> ETVQVNLPVSLEDLFVGKKKSFKIGRKGPHGASEKTQIDIQLKPGWKAGTKITYKNQGDYNPQ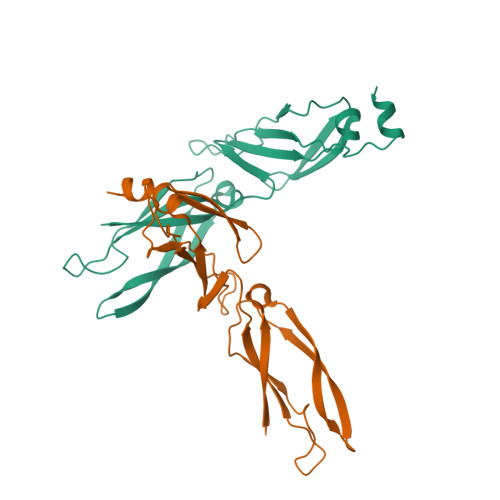TGRRKTLQFVIQEKSHPNFKRDGDDLIYTLPLSFKESLLGFSKTIQTIDGRTLPLSRVQPVQPSQTSTYPGQGMPTPKNPSQRGNLIVKYKVDYPISLNDAQKRAID> KVEDPKDFPVDLHAFLSQAVFSNRTVASFAVYTTKEKAQILYKKLMEKYSVTFISR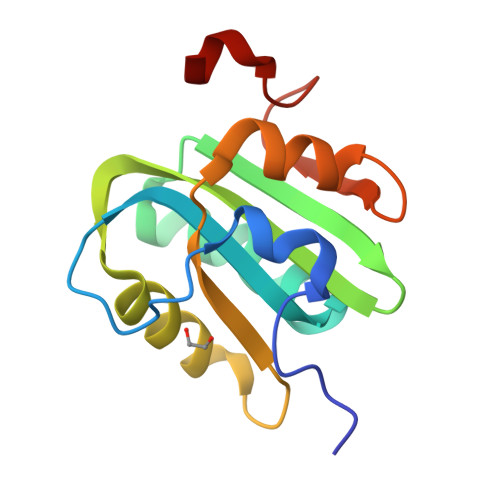HGFGGHNILFFLTPHRHRVSAINNYCQKLCTFSFLICKGVNKEYLFYSALCRQPYAVVEESIQGGLKEHDLNPE> APVNTTTEDETAQIPAEAVIGYSDLEGDFDVAVLPFSNSTNNGLLFINTTIASIAAKEEGVSLEKREAEAEFQSKDGVEDLDGPGDDLYVKDLSGCPGYKATKHWQTRSGFYADLTLAGPACNVFGTDLPDLKLEVEYQTSDRLHVKILDTNNTVYQ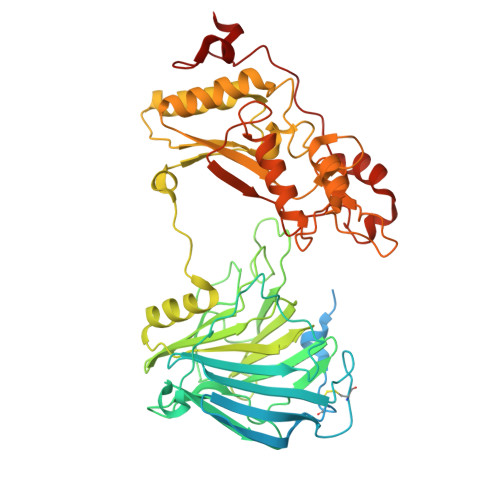VPDSVFPRPGFGEWCSPKDSKLKFDFQADPFSFTVSRTDTGEVLFDTTGNKLVFESQYVYLKTHLPQNPHLYGLGEHSDAFMLNTTNYTRTIYTRDAYGTPQGENLYGAHPIYFDHRQTGTHGVFLLNSNGMDIFIDNNATQYLEYNIIGGVLDFYFIAGPSPRDVAIQYAEITQTPLMTPYWGLGYHQCKYGYQDVYEVAAVVANYSTNNIPLETIWTDIDYMDRRRIFTIDPERFPANLYKDLVDTIHARDQHYIVMVDPAVYYKESNPALDEGLRYDIFMKENNGSEYQGVVWAGPSHFPDWFHPDSQQYWSEQFLAFFDGTNGPDIDALWIDMNEPANFYNRPYPGNNTTPENFAEVDGDPPAAPAVRDGPDAPIPGFPASLQPNWV> DVYQEPTDPKFPQQWYLSGVTQRDLNVKAAWAQGYTGHGIVVSILDDGIEKNHPDLAGNYDPGASFDVNDQDPDPQPRYTQMNDNRHGTRCAGEVAAVANNGVCGVGVAYNARIGGVRMLDGEVTDAVEARSL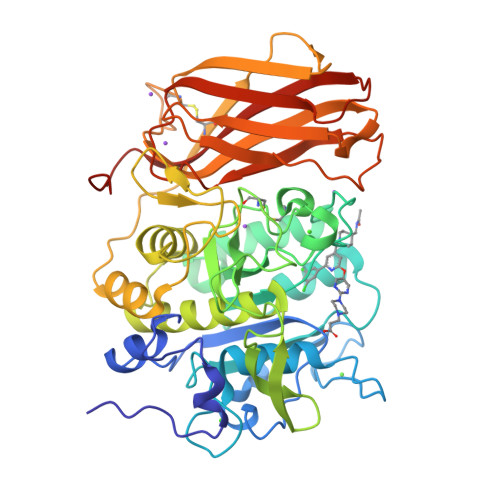GLNPNHIHIYSASWGPEDDGKTVDGPARLAEEAFFRGVSQGRGGLGSIFVWASGNGGREHDSCNCDGYTNSIYTLSISSATQFGNVPWYSEACSSTLATTYSSGNQNEKQIVTTDLRQKCTESHTGTSASAPLAAGIIALTLEANKNLTWRDMQHLVVQTSKPAHLNANDWATNGVGRKVSHSYGYGLLDAGAMVALAQNWTTVAPQRKCIIDILTEPKDIGKRLEVRKTVTACLGEPNHITRLEHAQARLTLSYNRRGDLAIHLVSPMGTRSTLLAARPHDYSADGFNDWAFMTTHSWDEDPSGEWVLEIENTSEANNYGTLTKFTLVLYGTASGSLVPRGSHHHH>[2x]GEFNTIQQLMMILNSASDQPSENLISYFNNCTVNPKESILKRVKDIGYIFKEKFAKAVGQGCVEIGSQRYKLGVRLYYRV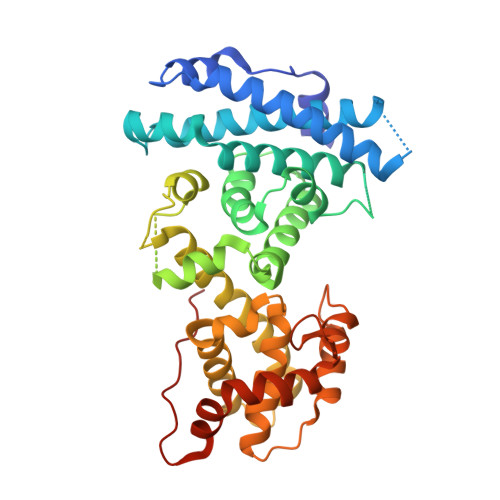MESMLKSEEERLSIQNFSKLLNDNIFHMSLLACALEVVMATYSRSTSQNLDSGTDLSFPWILNVLNLKAFDFYKVIESFIKAEGNLTREMIKHLERCKHRIMESLAWLSDSPLFDLIKQSKDREGPTDHLESACPLNLPLQNNHTAADMYLEPVRAPKKKSTSLSLFYKKVYRLAYLRLNTLCERLLSEHPELEHIIWTLFQHTLQNEYELMRDRHLDQIMMCSMYGICKVKNIDLKFKIIVTAYKDLPHAVQETFKRVLIKEEEYDSIIVFYNSVFMQRLKTNILQYASTRPPTLAPIPHIPRSPYKFP>[2x]MQSSTSTDQHVLHHMDPHRFTSQIPTATSSQLRRRNSTNQGLTDMINKSIARNTISGTGIPTGGINKNKRTRSTVAGGTNGTALALNDKSNSRNSVSRLSINQLGSLQQHLSNRDPRPLRDKNFQSAIQEEIYDYLKKNKFDIETNHPISIKFLKQPTQKGFIIIFKWLYLR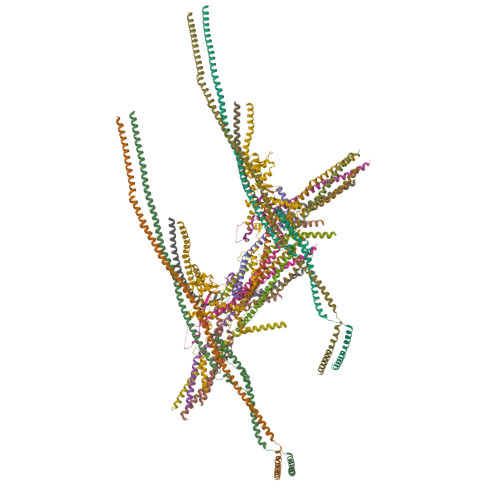LDPGYGFTKSIENEIYQILKNLRYPFLESINKSQISAVGGSNWHKFLGMLHWMVRTNIKLDMCLNKVDRSLINQNTQEITILSQPLKTLDEQDQRQERYELMVEKLLIDYFTESYKSFLKLEDNYEPSMQELKLGFEKFVHIINTDIANLQTQNDNLYEKYQEVMKISQKIKTTREKWKALKSDSNKYENYVNAMKQKSQEWPGKLEKMKSECELKEEEIKALQSNISELHKILRKKGISTEQFELQNQEREKLTRELDKINIQSDKLTSSIKSRKLEAEGIFKSLLDTLRQYDSSIQNLTRSRSQLGHNVNDSSLKINISENLLDRDFHEGISYEQLFPKGSGINESIKKSILKLNDEIQERIKTIEKDNITLEKDIKNLKHDINEKTQINEKLELELSEANSKFELSKQENERLLVAQRIEIEKMEKKINDSNLLMKTKISDAEELVTSTELKLEELKVDLNRKRYKLHQQVIHVIDITSKFKINIQSSLENSENELGNVIEELRNLEFETEHNVTN;>MSRNQDVFPILDLQELVICLQSCDFALATQENISRPTSDYMVTLYKQIIENFMGISVESLLNSSNQETGDGHLQEENENIYLDTLNVLVLNKICFKFFENIGVQDFNMTDLYKPEAQRTQRLLSAVVNYARFREERMFDCNSFILQMESLLGQLRSKFDDYNLIQQQLKQYEDVDGDNIPDEQELQKLEEQNKELEIQLKKLTKIQETLSIDYNDYKISKQSIFKDLEALSFQIVELESNRDKLIKISNTDMEELSEGIKELNDLLIQRKKTLDDLTAQQKNLQDTVTTFETIISELYDVLRIISSEVQESNRTETELVGLKQNLINNKLKLMNVLETGIMYKLEILQEQLDLQLKNLEKLSQDTKEESRLNDTKLMDLQIKYENEIKPKIDKTDIFIQEELISGKINKLNDEIKQLQKDFEVEVKEIEIEYSLLSGHINKYMNEMLEYMQ[2x];>[3x]MSEDKAKLGTTRSATEYRLSIGSAPTSRRSSMGESSSLMKFADQEGLTSSVGEYNENTIQQLLLPKIRELSDSIITLDSNFTRLNFIHESLADLNESLGSLLYGIMSNSWCVEFSQAPHDIQDDLIAIKQLKSLEDEKNNLVMELSNMERGIKRKKDEQGENDLAKASQNKQFNQPLFPSSQVRKYRSYDNRDKRKPSKIGNNLQVENEEDYEDDTSSEASFVLNPTNIGMSKSSQGHVTKTTRLNNNTNSKLRRKSILHTIRNSIASGADLPIENDNVVNLGDLHPNNRISLGSGAARVVNGPVTKNRNSMFSGRAERKPTESRHSVAKKTEKKINTRPPFR;>[2x]MSEQSQLDDSTIDKLIPQIFNEMRSNLNNTTNKFPKSTGGGASDNISANSNSIRSFNSITTQSLLKESESLDKITAMIKNVTAALKNNLPVYVNQVHEVCKSTNSILDSWINIHSQAGYIHKLMSDQTYLKLINDRLHNENVNTNDEDGSTLHNVIALKKKEILDLRQKLENRKGEKDAAPAKPPNQGLNPRYGVQSGRRPVPSAGISNNGRVRKTHVPASKRPSGIPRVTNRWTKPTASSSRKMFR;>[2x]MDSIDEQIAIKRKELQSLQKITSLTDGLKIQLTELNEQIKEMGMNADSVAQLMNNWDSIINNISQASLGLLQYAEGDYEIGPWKDSKKKESEQSNETGLEAQENDKNDEDNDEDEDLVPLPETMVRIRVDGNE;>MMASTSNDEEKLISTTDKYFIEQRNIVLQEINETMNSILNGLNGLNISLESSIAVGREFQSVSDLWKTLYDGLESLSDEAPIDEQPTLSQSKTK[2x];>[2x]MENPHEQVQANILSRIIGNVKRLNESVAILNQELVTINNRNKNLEIMGAICDNYHSSVQFNLEATNNKKPPL;>[2x]MEHNLSPLQQEVLDKYKQLSLDLKALDETIKELNYSQHRQQHSQQETVSPDEILQEMRDIEVKIGLVGTLLKGSVYSLILQRKQEQESLGSNSK;>[2x]MGESLDRCIDDINRAVDSMSTLYFKPPGIFHNAILQGASNKASIRKDITRLIKDCNHDEAYLLFKVNPEKQSVSRRDGKEGVFDYVIKRDTDMKRNRRLGRPGEKPIIHVPKEVYLNKDRLDLNNKRRRTATTSGGGLNGFIFDTDLIGSSVISNSSSGTFKALSAVFKDDPQIQRLLYALENGSVLMEEESNNQRRKTIFVEDFPTDLILKVMAEVTDLWPLTEFKQDYDQLYHNYEQLSSKLRFIKKEVLLQDDRLKTMSQYHPSSSHDVAKIIRKEKDEIRRLEMEIANLQE;>MDSASKEETLEKLDQEITVNLQKIDSNLSFCFHKITQDIIPHVATYSEICERIMDSTEWLGTMFQETGLVNLQANAAAPVGNAPVKSLVSNNVGIFPTSAEEASRQSQTDNGPNEADSAVHVNRDVHSMFNNDSIDDFHTANITSTGQILKLPDSSDEDTGSEAVPSREQTDLTGEGHGGADDEQDESTIQRQSRKRKISLLLQQQYGSSSSMVPSPIVPNKMRKQLAHEEHINNDGDNDDENSNNIESSPLKQGHHHPKGQADDNNEGPDEEESTKEVPKPGTIIHFSTNR[2x];>MNANKQRQYNQLAHELRELQTNLQETTKQLDIMSKQCNENLVGQLGKVHGSWLIGSYIYYMEQMLGKTQ[2x];>MTDALEQSVLALEGTVSVLKDSVESLKCANEPSTNLASTMLQTKRVFRLVPEYDVERSKLDLIEEVEPLVRTLGDKLRKSMGRMQRELDTLQQTYELNDLRLKKNISMDDDDALNSPDMGQEYEGRDADDVVMMASSTNEELEELKKLKEKKKQLENKLEILKQK[2x]> MSILTRWLLIPPVNARLIGRYRDYRRHGASAFSATLGCFWMILAWIFIPLEHPRWQRIRAEHKNLYPHINASRPRPLDPVRYLIQTCWLLIGASRKETPKPRRRAFSGLQNIRGRYHQWMNELPERVSHKTQHLDEKKELGHLSAGARRLILGIIVTFSLILALICVTQPFNPLAQFIFLMLLWGVALIVRRMPGRFSALMLIVLSLTVSCRYIWWRYTSTLNWDDPVSLVCGLILLFAETYAWIVLVLGYFQVVWPLNRQPVPLPKDMSLWPSVDIFVPTYNEDLNVVKNTIYASLGIDWPKDKLNIWILDDGGREEFRQFAQNVGVKYIARTTHEHAKAGNINNALKYAKGEFVSIFDCDHVPTRSFLQMTMGWFLKEKQLAMMQTPHHFFSPDPFERNLGRFRKTPNEGTLFYGLVQDGNDMWDATFFCGSCAVIRRKPLDEIGGIAVETVTEDAHTSLRLHRRGYTSAYMRIPQAAGLATESLSAHIGQRIRWARGMVQIFRLDNPLTGKGLKFAQRLCYVNAMFHFLSGIPRLIFLTAPLAFLLLHAYIIYAPALMIALFVLPHMIHASLTNSKIQGKYRHSFWSEIYETVLAWYIAPPTLVALINPHKGKFNVTAKGGLVEEEYVDWVISRPYIFLVLLNLVGVAVGIWRYFYGPPTEMLTVVVSMVWVFYNLIVLGGAVAVSVESKQVRRSHRVEMTMPAAIAREDGHLFSCTVQDFSDGGLGIKINGQAQILEGQKVNLLLKRGQQEYVFPTQVARVMGNEVGLKLMPLTTQQHIDFVQCTFARADTWALWQDSYPEDKPLESLLDILKLGFRGYRHLAEFAPSSVKGIFRVLTSLVSWVVSFIPRRPERSETAQPSDQALAQQGSARSSGRTGLEFEEFYPYDVPDYAADYKDDDDKRS;> MKRKLFWICAVAMGMSAFPSFMTQATPATQPLINAEPAVAAQTEQNPQVGQVMPGVQGADAPVVAQNGPSRDVKLTFAQIAPPPGSMVLRGINPNGSIEFGMRSDEVVTKAMLNLEYTPSPSLLPVQSQLKVYLNDELMGVLPVTKEQLGKKTLAQMPINPLFITDFNRVRLEFVGHYQDVCENPASTTLWLDVGRSSGLDLTYQTLNVKNDLSHFPVPFFDPRDNRTNTLPMVFAGAPDVGLQQASAIVASWFGSRSGWRGQNFPVLYNQLPDRNAIVFATNDKRPDFLRDHPAVKAPVIEMINHPQNPYVKLLVVFGRDDKDLLQAAKGIAQGNILFRGESVVVNEVKPLLPRKPYDAPNWVRTDRPVTFGELKTYEEQLQSSGLEPAAINVSLNLPPDLYLMRSTGIDMDINYRYTMPPVKDSSRMDISLNNQFLQSFNLSSKQEANRLLLRIPVLQGLLDGKTDVSIPALKLGATNQLRFDFEYMNPMPGGSVDNCITFQPVQNHVVIGDDSTIDFSKYYHFIPMPDLRAFANAGFPFSRMADLSQTITVMPKAPNEAQMETLLNTVGFIGAQTGFPAINLTVTDDGSTIQGKDADIMIIGGIPDKLKDDKQIDLLVQATESWVKTPMRQTPFPGIVPDESDRAAETRSTLTSSGAMAAVIGFQSPYNDQRSVIALLADSPRGYEMLNDAVNDSGKRATMFGSVAVIRESGINSLRVGDVYYVGHLPWFERLWYALANHPILLAVLAAISVILLAWVLWRLLRIISRRRLNPDNE;>MASWSHPQFEKGSMRDIVDPVFSIGISSLWDELRHMPAGGVWWFNVDRHEDAISLANQTIASQAETAHVAVISMDSDPAKIFQLDDSQGPEKIKLFSMLNHEKGLYYLTRDLQCSIDPHNYLFILVCANNAWQNIPAERLRSWLDKMNKWSRLNHCSLLVINPGNNNDKQFSLLLEEYRSLFGLASLRFQGDQHLLDIAFWCNEKGVSARQQLSVQQQNGIWTLVQSEEAEIQPRSDEKRILSNVAVLEGAPPLSEHWQLFNNNEVLFNEARTAQAATVVFSLQQNAQIEPLARSIHTLRRQRGSAMKILVRENTASLRATDERLLLACGANMVIPWNAPLSRCLTMIESVQGQKFSRYVPEDITTLLSMTQPLKLRGFQKWDVFCNAVNNMMNNPLLPAHGKGVLVALRPVPGIRVEQALTLCRPNRTGDIMTIGGNRLVLFLSFCRINDLDTALNHIFPLPTGDIFSNRMVWFEDDQISAELVQMRLLAPEQWGMPLPLTQSSKPVINAEHDGRHWRRIPEPMRLLDDAVERSS[2x];>MMTISDIIEIIVVCALIFFPLGYLARHSLRRIRDTLRLFFAKPRYVKPAGTLRRTEKARATKK[2x];>MTQFTQNTAMPSSLWQYWRGLSGWNFYFLVKFGLLWAGYLNFHPLLNLVFAAFLLMPLPRYSLHRLRHWIALPIGFALFWHDTWLPGPESIMSQGSQVAGFSTDYLIDLVTRFINWQMIGAIFVLLVAWLFLSQWIRITVFVVAILLWLNVLTLAGPSFSLWPAGQPTTTVTTTGGNAAATVAATGGAPVVGDMPAQTAPPTTANLNAWLNNFYNAEAKRKSTFPSSLPADAQPFELLVINICSLSWSDIEAAGLMSHPLWSHFDIEFKNFNSATSYSGPAAIRLLRASCGQTSHTNLYQPANNDCYLFDNLSKLGFTQHLMMGHNGQFGGFLKEVRENGGMQSELMDQTNLPVILLGFDGSPVYDDTAVLNRWLDVTEKDKNSRSATFYNTLPLHDGNHYPGVSKTADYKARAQKFFDELDAFFTELEKSGRKVMVVVVPEHGGALKGDRMQVSGLRDIPSPSITDVPVGVKFFGMKAPHQGAPIVIEQPSSFLAISDLVVRVLDGKIFTEDNVDWKKLTSGLHKQHRSPRTQMQ[3x];>MAVLGLQGVRGGVGTTTITAALAWSLQMLGENVLVVDACPDNLLRLSFNVDFTHRQGWARAMLDGQDWRDAGLRYTSQLDLLPFGQLSIEEQENPQHWQTRLSDICSGLQQLKASGRYQWILIDLPRDASQITHQLLSLCDHSLAIVNVDANCHIRLHQQALPDGAHILINNFRIGSQVQDDIYQLWLQSQRRLLPMLIHRDEAMAECLAAKQPVGEYRSDALAAEEILTLANWCLLNYSGLKTPVGSKS[2x];>[2x]MGSSHHHHHHHHAAGSNNNEPDTLPDPAIGYIFQNDIVALKQAFSLPDIDYADISQREQLAAALKRWPLLAEFAQQK

Bacterial cellulosic polymers constitute a prevalent class of biofilm matrix exopolysaccharides that are synthesized by several types of bacterial cellulose secretion (Bcs) systems, which include conserved cyclic diguanylate (c-di-GMP)-dependent cellulose synthase modules together with diverse accessory subunits. In E. coli, the biogenesis of phosphoethanolamine (pEtN)-modified cellulose relies on the BcsRQABEFG macrocomplex, encompassing inner-membrane and cytosolic subunits, and an outer membrane porin, BcsC. Here we present cryo-EM structures of the E. coli Bcs macrocomplex positioning all seven BcsRQABEFG partners and multiple c-di-GMP-binding sites.

To gain mechanistic insights into the c-di-GMP-dependent regulation, we kept low micromolar concentrations of the dinucleotide (2–4 µM) throughout the purification procedure and prepared the cryogrids after a final fast concentration step to ∼2:1 c-di-GMP:Bcs macrocomplex ratio. Interestingly, the remaining particles showed a c-di-GMP-free BcsA synthase and a more extended vestibule conformation, where the central BcsEREC* domains engage in a different dimerization interface mediated by the pairs of β1–β2 connecting loops (melted α1 relative to canonical response regulators) and the C-proximal α-helices (canonical α5). Densities for the PilZ-proximal GGDEF* domain feature markedly lower-resolution, however, the conformation for both BcsEREC*-GGDEF* tandems is still consistent with the closed BcsE state and intercalated c-di-GMP complexation. The overall BcsE fold features a more extended conformation along the NTPase*-REC* domain linkers, neither BcsE protomer contacts the cytosolic synthase modules and the X-shaped BcsF dimer is found shifted near the fifth and fourth BcsB protomer as opposed to the c-di-GMP-saturated complex shown above. Nevertheless, the BcsRQ tandem is retained as an apical complex and the synthase-proximal BcsQ and BcsR protomers engage in similarly extensive contacts with the catalytic and PilZ modules. The latter is only partially rotated around the hinge helix relative to the c-di-GMP-bound state (12.8° rotation and 1.7 Å displacement) and the N-proximal PilZ domain linker is partially unstructured but remains far from gating loop-stabilizing interactions with the BcsAGT core. Although this vestibule is observed in two discreet c-di-GMP-bound conformations dependent on dinucleotide abundance and stabilizing BcsB-BcsF interactions, BcsA remains BcsRQ-bound and, as a result, presents a catalytically competent conformation even in the absence of direct dinucleotide complexation. We further demonstrate that BcsE, a secondary c-di-GMP sensor, can remain dinucleotide-bound and retain the essential-for-secretion BcsRQ partners onto the synthase even in the absence of direct c-di-GMP-synthase complexation, likely lowering the threshold for c-di-GMP-dependent synthase activation.>MAWNNIVFYSLGDVNSYQGGNVVITQRPQFITSWRPGIATVTWNQCNGPEFADGSWAYYREYIAWVVFPKKVMTKNGYPLFIEVHNKGSWSEENTGDNDSYFFLKGYKWDQRAFDTANLCQKPGETTRLTEKFDDIIFKVALPADLPLGD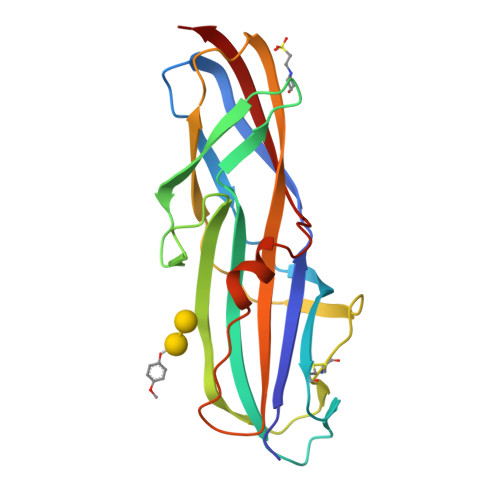YSVTIPYTSGIQRHFASYLGARFKIPYNVAKTLPRENEMLFLFKNIGG[2x]>MTTVYYDQDVKTDALQGKKIAVVGYGSQGHAHAQNLKDNGYDVVIGIRPGRSFDKAKEDGFDVFPVAEAVKQADVIMVLLPDEIQGDVYKNEIEPNLEKHNALAFAHGFNIHFGVIQPPADVDVFLVAPKGPGHLVRRTFVEGSAVPSLFGIQQDASGQARNIALSYAKGIGATRAGVIETTFKEETETDLFGEQAVLCGGVSKLIQSGFETLVEAGYQPELAYFEVLHEMKLIVDLMYEGGMENVRYSISNTAEFGDYVSGPRVITPDVK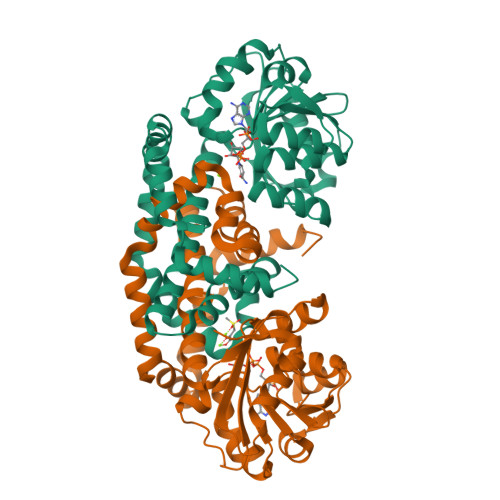ENMKAVLTDIQNGNFSNRFIEDNKNGFKEFYKLREEQHGHQIEKVGRELREMMPFIKSKSIEK[2x]>TPEGLSSEQQRAFLAVTQTPHPAHLITGPAGTGKTTLLYALQEFYKGRAVTLAPTGTAALQARGQTVHSFFRFPARLLRYRHPEDIRPPGPHSPLRKAIEQMEVLILDEVGMVRVDLLEAMDWALRKTRKRLEEPFGGVKVLLLGDTRQLEPVVPGGEEALYIARTWGGPFFFQAHVWEEVALRVHRLWESQRQREDPLFAELLKRLRQGDPQALETLNRAAVRPDGGEEPGTLILTPRRKEADALNLKRLEALPGKPLEYQAQVKGEFAETDFPTEAALTLKKGAQVILLRNDPLGEYFNGDLGWVEDLEAEALAVRLKRNGRRVVIRPFVWEKIVYTYDSEREEIKPQVVGTFRQVPVRLAWALTVHKAQGLTLDKVHLELGRGLFAHGQL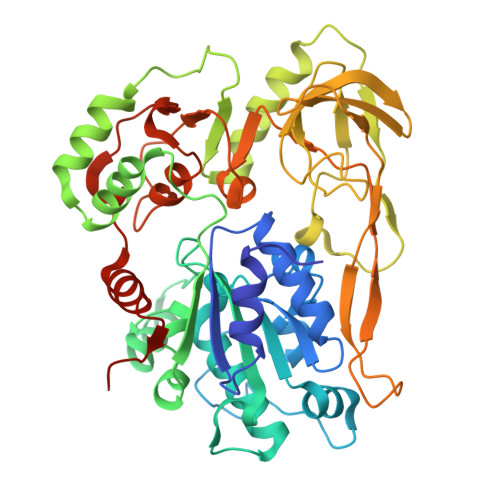YVALTRVRRLQDLSLSRPIAPTELLWRPEVEVFETRIQEGIWQKSHGWPSL[2x]>GHMRGCTVWLTGLSGAGKTTVSMALEEYLVCHGIPCYTLDGDNIRQGLNKNLGFSPEDREENVRRIAEVAKLFADAGLVCITSFISPYTQDRNNARQIHEGASLPFFEVFVDAPLHVCEQRDVKGLYKKARAGEIKGFTGIDSEYEKPEAPELVLKTDSCDVNDCVQ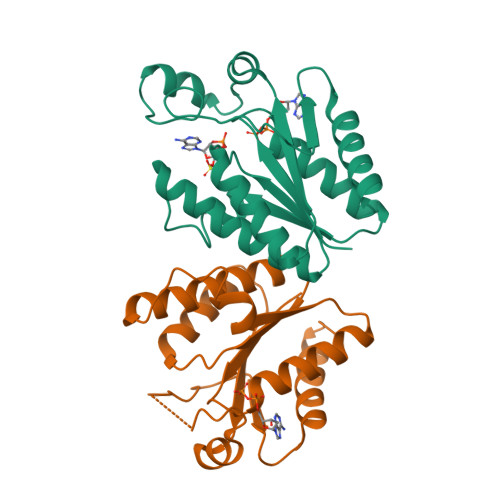QVVELLQERDIV[2x]>[2x]AEETCFDKYTGNTYRVGDTYERPKDSMIWDCTCIGAGRGRISCTIANRC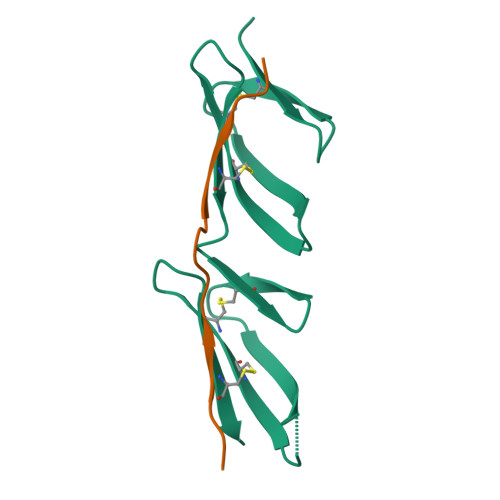HEGGQSYKIGDTWRRPHETGGYMLECVCLGNGKGEWTCKPI;>XKGIVTGAVSDHTTVEDTKX[2x]> MPLTEIQVESYKKALQADVPPEKRENVGIQAAFKETFPIEEGDKGKGGLVLDFLEYRIGDPPFSQDECREKDLTYQAPLYARLQLIHKDTG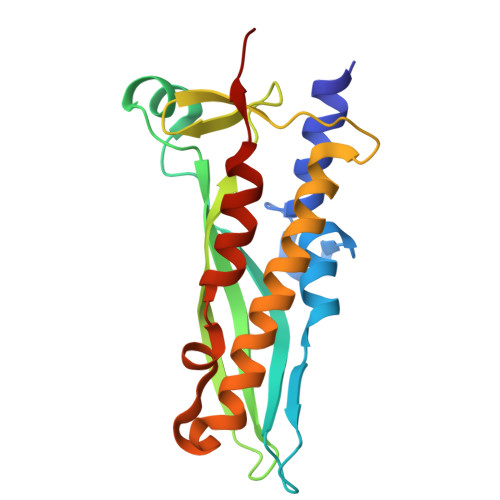LIKEDEVFLGHLPLMTEDGSFIINGADRVIVSQGGRTVGELMADQFRVGLARLARGVRERMVMGSPDTLTPAKLVNSRPLEAALREFFSRSQLSQFK> MKTMRKQIYKKAYWLLLPFLPLALANTFLVKEDSKNVTAYTPFATPITDSKSDLVSLAQLDSSYQIADQTIHNTNLFVLFKSRDVKVKYESSGSNNISFDSTSQGEKPSYVVEFTNSTNIGIKWTMVKKYQLDVPNVSSDMNQVLKNLILEQPLTKYTLNSSLAKEKGKTQREVHLGSGQANQWTSQRNQHDLNNNPSPNASTGFKLTTGNAYRKLSESWPIYEPIDGTKQGKGKDSSGWSSTEEN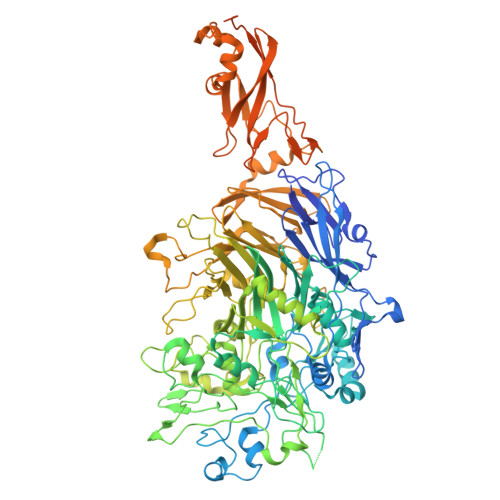EAKNDAPSVSGGGSSSGTFNKYLNTKQALESIGILFDDQTPRNVITQLYYASTSKLAVTNNHIVVMGNSFLPSMWYWVVERSAQENASNKPTWFANTNLDWGEDKQKQFVENQLGYKETTSTNSHNFHSKSFTQPAYLISGIDSVNDQIIFSGFKAGSVGYDSSSSSSSSSSSSTKDQALAWSTTTSLDSKTGYKDLVTNDTGLNGPINGSFSIQDTFSFVVPYSGNHTNNGTTGPIKTAYPVKKDQKSTVKINSLINATPLNSYGDEGIGVFDALGLNYNFKSNQERLPSRTDQIFVYGIVSPNELRSAKSSADSTGSDTKVNWSNTQSRYLPVPYNYSEGIIDADGFKRPENRGASVTTFSGLKSIAPDGFANSIANFSVGLKAGIDPNPVMSGKKANYGAVVLTRGGVVRLNFNPGNDSLLSTTDNNIAPISFSFTPFTAAESAVDLTTFKEVTYNQESGLWSYIFDSSLKPSHDGKQTPVTDNMGFSVITVSRTGIELNQDQATTTLDVAPSALAVQSGIQSTTQTLTGVLPLSEEFSAVIAKDSDQNKIDIYKNNNGLFEIDTQLSNSVATNNGGLAPSYTENRVDAWGKVEFADNSVLQARNLVDKTVDEIINTPEILNSFFRFTPAFEDQKATLVATKQSDTSLSVSPRIQFLDGNFYDLNSTIAGVPLNIGFPSRVFAGFAALPAWVIPVSVGSSVGILFILLVLGLGIGIPMYRVRKLQDASFVNVFKKVDTLTTAVGSVYKKIITQTGVVKKAPSALKAANPSVKKPAAFLKPPVQPPSKPEGEQKAVEVKSEETKSHHHHHH(2E)-3-{6-[(1S)-1-(3-amino-2,6-dichlorophenyl)ethoxy]-4-cyclopropylquinolin-3-yl}prop-2-enoic acid 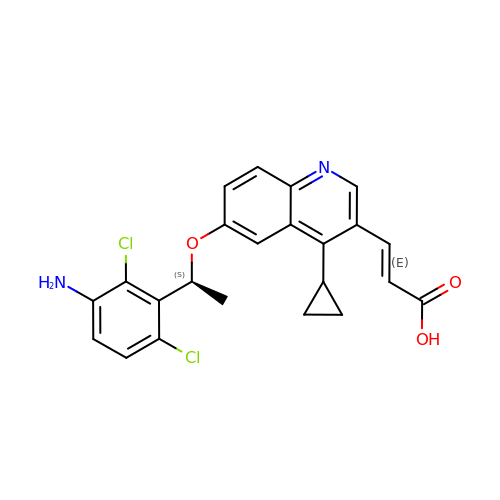| C23 H20 Cl2 N2 O3 | XJXAZWMUTUJRMD-KFRNIWOLSA-N>MPERITLYTAKICPFAQRVEIALHEAKAHHNVEQFQIDLQNKPEWYAPKVNPASKVPAIAYGGPHVPPDQPSPESIKLAESLILVEFVADLFPHSHLLPHDPVKRAQARFFIDGVSTKFIPAWHAFSQGKSSEEDFLTAVEHLQALLPESGFAVGAYSIADVALTPFLGRARVTLKEDLGGYPRGEGPRVLAVLTSGTGRLARFGKYAQDLLARESFQATFDEAYITERYKARFADLRKH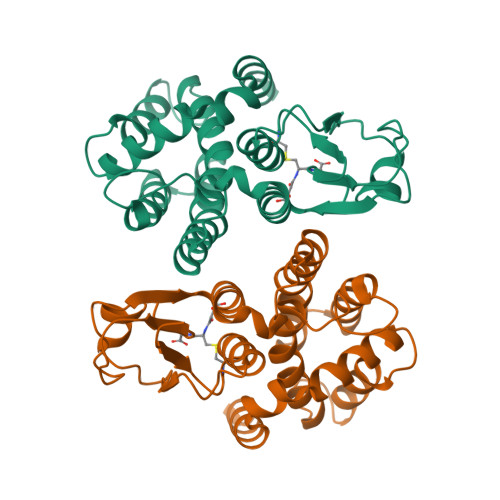HHHHH[2x]ADO, a ferrous ion [Fe(II)]–dependent thiol dioxygenase, uses O2 to oxidize both the namesake small-molecule and cysteine-derived thiol groups in proteins, as elaborated below. Furthermore, ADO also transduces targeted oxygen-dependent degradation of important regulatory proteins with N-terminal cysteine residues, following removal of genetically encoded N termini. Here, we identify 2-aminoethanethiol dioxygenase (ADO), a key mediator of targeted protein degradation, as a selective HYZ target. The drug chelates ADO’s metallocofactor and can alkylate one of its ligands.

The HYZyne-ADO adduct isolated from cells has lost the hydrazine moiety of the probe. The most likely mechanisms for the implied C-N fragmentation involve nitrogen-centered radical generation. Thus, the initial step is likely to involve coordination to and activation by the metal center, analogously to the mechanism by which the substrate is oxidized. To capture the anticipated initial state of the HYZ•ADO reaction in vitro, we first purified and crystallized the Fe(II)•ADO complex as previously described. Thus, the Fe(II) crystals did not capture the expected prereaction complex. However, attempts to identify conditions that recapitulate covalent coupling to ADO in vitro were unsuccessful, and we posit that a reactant is likely to be present in vivo that is needed to oxidize the drug to initiate its decomposition.

> GHMASPRDNMASLIQRIARQASLTFRGSGGGRGASDRDAASGPEAPMQPGFPENLSKLKSLLTQLRAEDLNIAPRKATLQPLPPNLPPVTYMHIYETDGFSLGVFLLKSGTSIPLHDHPGMHGMLKVLYGTVRISCMDKLDAGGGQRPRALPPEQQFEPPLQPREREAVRPGVLRSRAEYTEASGPCILTPHRDNLHQIDAVEGPAAFLDILAPPYDPDDGRDCHYYRVLEPVRPKEASSSASDLPREVWLLETPQADDFWCEGEPYPGPKVFP> RRCVMAKGEDPAHVAGWDDRQDAVEWWWTEANDSRGRQRLEAAAAVAAAAASSTVGLPLFPRFSPGRRRRRRPPAPPPPPPPLFLSRHLHSMPWLWCTCVKMQMYYTPTALTCPLSNSLAAHVGHIIVGVAALLPYSMLLFLTVMCNPRKHEPVLRAQRIRWLTFHSLMFRLLRCITASPAVAASVAVAAAQTPTSLRPAAVCRRGVHLAPSVLAASAPPPPPQQQQQPTSAAVPASTATSTTTIAAGPYRRVGNVFIVTCIDHPFKFSWEVNRMLRELRLEFMGQTTVVPDIPPVRKRIWRVRHVVRVDQLDLDEAKALIGIPEHISFRDLAGQIPPTFGRGGSVANPHMRSKMNFMRLRRMRLRDVMHRDQLEKRLLEERHHALQQQQ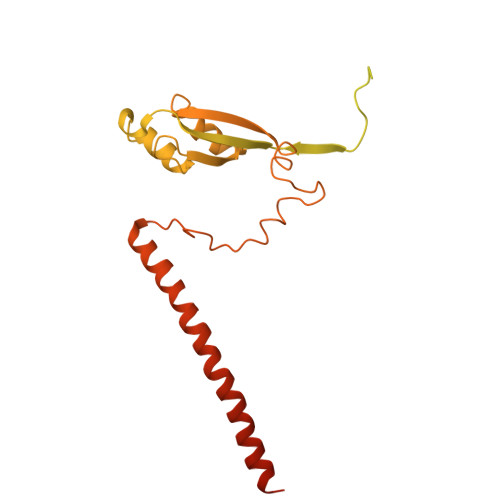QQQQGGGEAAAAAAATTA> MRWYPWLRPDFEKLVASYQAGRGHHALLIQALPGMGDDALIYALSRYLLC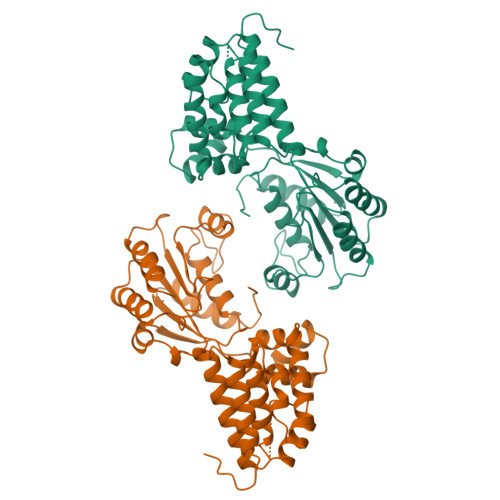QQPQGHKSCGHCRGCQLMQAGTHPDYYTLAPEKGKNTLGVDAVREVTEKLNEHARLGGAKVVWVTDAALLTDAAANALLKTLEEPPAETWFFLATREPERLLATLRSRCRLHYLAPPPEQYAVTWLSREVTMSQDALLAALRLSAGSPGAALALFQGDNWQARETLCQALAYSVPSGDWYSLLAALNHEQAPARLHWLATLLMDALKRHHGAAQVTNVDVPGLVAELANHLSPSRLQAILGDVCHIREQLMSVTGINRELLITDLLLRIEHYLQPGVVLPVPHL>[2x]FPRVSQELKTALSTLQQTFVV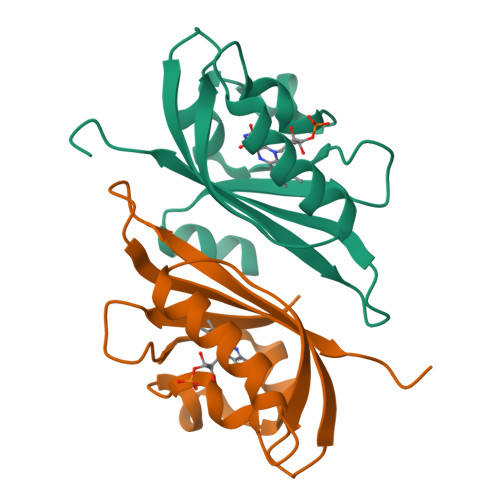SDATQPHCPIVYASSGFFTMTGYSSKEIVGRNCRFLQGPDTDKNEVAKIRDCVKNGKSYCGRLLNYKKDGTPFWNLLTVTPIKDDQGNTIKFIGMQVEVSKYTEGVNDK> MSKFSESTLSGWTKPASVTEEDRIENTISMIKSAIKNDNNFDNLVYEVFVQGSYGNNTNVRTNSDIDVNIMLTSTFYSKYPEGKTNSDYGFTDGTITYNEYKNLILTALTNKFGTGNVTVGNKSIKITSNSYRVEADCIPSLLYRNYEYENSSSPNNYIEGIKYFASDNTSVVNYPKVHINNGIEKNNQTHKNYKRLVRVIKRLRNKMTAENHFTNENITSFLIECLIWNVPNNYINDYDTWDETIKQTLIFIKSSINDNSYKNWTEVSGMFYLFHNNRKWTSDDVSSFV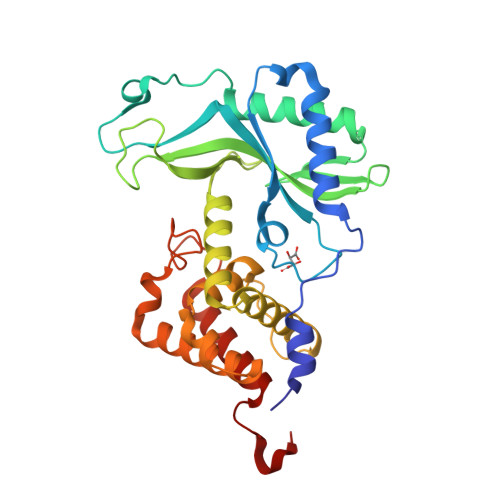NSLWSFMEYLEHHHHHH>STSDGDDLFVPVSNFDPKSIFPEIKHPFEPMYANTENGKIVPTNSWISNLFYPSADNLAPTTPDPYTLRLLDGYGGNPGLTIRQPSAKVLGSYPPTNDVPYTDAGYMINSVVVDLRLTSSEWSDVVPDRQVTDWDHLSANLRLSTPQDSNSYIDFPIVRGMAYITANYNNLTPQFLSQHAIISVEADEKKSDDNTSTFSGRKFKITMNDDPTSTFIIYSLGDKPLELRKQDNSNLVASKPYTGVIRVAKLPAPEFETLLDASRAVWPTGGDISARSDDNNGASYTIKWKTNSNEAPLLTYAYAHHLTSIDDSNVKRTDMTLQSATKGPMTALVGNEWTLRETELSPVEWLPLQAAPNPTTINEIMTEINKDIASNYTQETAKEDNYFSGKGLQKFAMLALILNKSDQTQLRNPELAQIALDKLKAAFLPYLQNEQADPFRYDTLYKGIVAKAGLPTSMGGTDDLSAEFGHSYYSDHHYHQGYFVVTAAIIHHLDPTWNADRLKAWTEALIRDVNNANDGDEYFAAFRNWDWFAGHSWAGGIKPDGALDGRDQESVPESVNFYWGAKLWGLATGNTPLTKLASLQLAVTKRTTYEYFWMLDGNKNRPENIVRNKVIGIYFEQKTDYTTYFGRFLEYIHGIQQLPMTPELMEYIRTPEFVSQEWDEKLGAIAPTVQSPWAGVLYLNYAIINPAEAYPALRKVQMDDGQTRSYSLYLTATRPHFFRRSLLAALARHGSTRR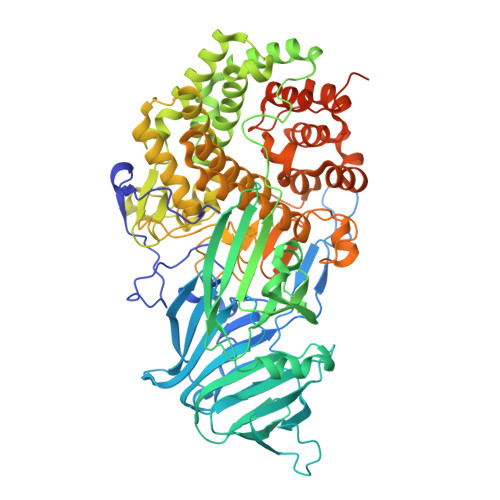PSLPSSGDDDKHEDGFLLRFRRLNPFNLKHRIY[2x]>[4x]MLKGKV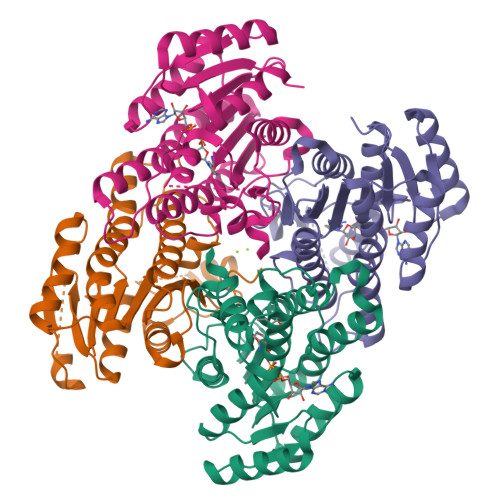AVVTGSTSGIGLGIATALAAQGADIVLNGFGDAAEIEKVRAGLAAQHGVKVLYDGADLSKGEAVRGLVDNAVRQMGRIDILVNNAGIQHTALIEDFPTEKWDAILALNLSAVFHGTAAALPHMKKQGFGRIINIASAHGLVASANKSAYVAAKHGVVGFTKVTALETAGQGITANAICPGWVRSPLVEKQISALAEKNGVDQETAARELLSEKQPSLQFVTPEQLGGTAVFLASDAAAQITGTTVSVDGGWTAR N-[(1S,2S,4R)-2-HYDROXY-1-ISOBUTYL-5-({(1S)-1-[(ISOPROPYLAMINO)CARBONYL]-2-METHYLPROPYL}AMINO)-4-METHYL-5-OXOPENTYL]-5-[METHYL(METHYLSULFONYL)AMINO]-N'-[(1R)-1-PHENYLETHYL]ISOPHTHALAMIDE | C36 H55 N5 O7 S | 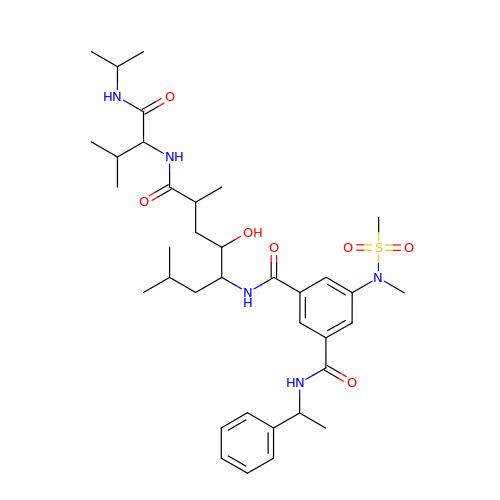BJOCXJJVELLFKM-LLWRDSBASA-N N-[(E)-2-AMINO-1-(3-{[AMINO(IMINO)METHYL]AMINO}PROPYL)-2-HYDROXYVINYL]BENZAMIDE 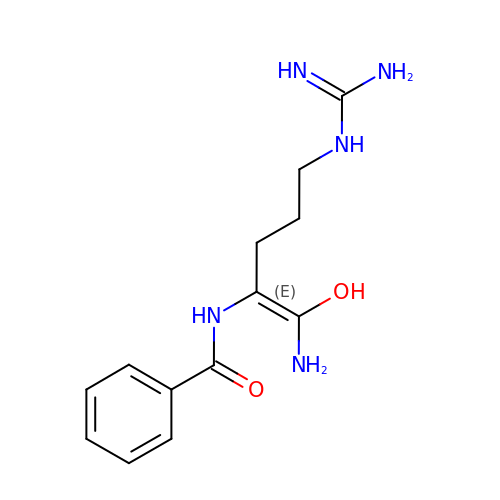| C13 H19 N5 O2 | YRINIXCRGISJPA-UHFFFAOYSA-N9-(3-PHENYLMETHYLAMINO)-1,2,3,4-TETRAHYDROACRIDINE 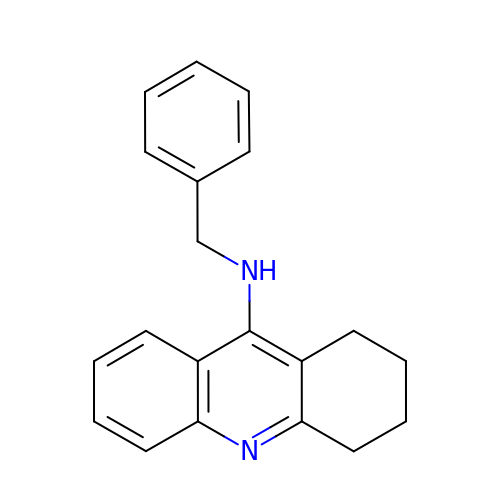| C20 H20 N2 | JYJAEHAURXXPSD-UHFFFAOYSA-N> MHAVSVGKGSYATEFPEIDFGGINDPGFRDQQGEPPATIYRSDRVTGPMQTNSWWGSLAVDRFSMNQYPHPFSVRHRAEGLHVFYDAPHNMVVHENREAGTWHIHGAIGTDFTIKHSGTANFEQAVVDDYNDWYVRGLLENGAHQMAITYGVGSPYIFVEYEDGSAVLDFDIAPDVWEMNGHVIGFSTHDHKHYAAFAPPGQNWSGIGSKTLTNNADYIAIAKLPEKDGNMLAKFEQYAYSVVRDAVADWTYDEATGTVTTTFEVTTEAKVQGAPDGTIFALYPHQYRHLASSSENQLLQNYQYEIIRGTMIGLEGKRFTTELTYPGVLPSLPDLGDYDRERLIGYLHDATSDYPTGSDTYELGKYIGKLATLAPIADQMGEYELAEQFRGELKDILEDWLQATNASGQLKGKNLFYYNENWGTILGYHAAHSSATRINDHHFHYGYFVKAAAEIARADQEWAKSENWGGMIDLLIRDFMADRDDDLFPYLRMFDPYSGNSWADGLATFDAGNNQQSSSEAMHAW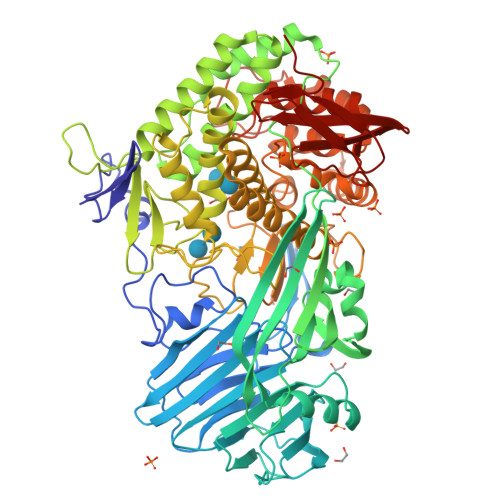TNVILWAEATGNKALRDRAIYLYTTEMSAINEYFFDVHQEIFPEEYGPEIVTINWGGKMDHATWWNSGKVEKYAINWLPFHGGSLYLGHHPDYVDRAYEELRRDIGSTDWNLWSNLVWMYRAFTNPDDALQQMEASIDDYGLFDPGNEKIIERGSTKAQTYHWIHNLAELGRVDPTVTANHPIYAVFNKNGNRTYIVYNFSDSPITVQFSDGHSIQVEPHSFNIGNGD> GYSDDEEEESNAINVVSEKTKSLEEKIAYYKMKGHTERGYITIYTNLGDFEVELYWYHSP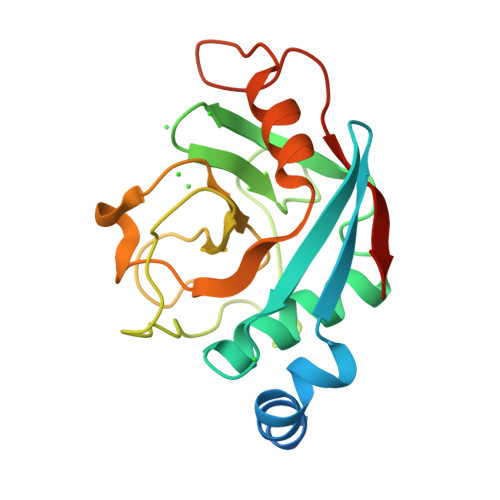KTCLNFYTLCEMGFYDNTIFHRVIPNFVIQGGDPTGTGKGGKSIYGEYFEDEINKELKHTGAGILSMSNNGPNTNSSQFFITLAPLPHLDGKHTIFARVSKNMTCIENIASVQTTATNKPIFDLKILRTSTAVNAD>MEAGITGTWY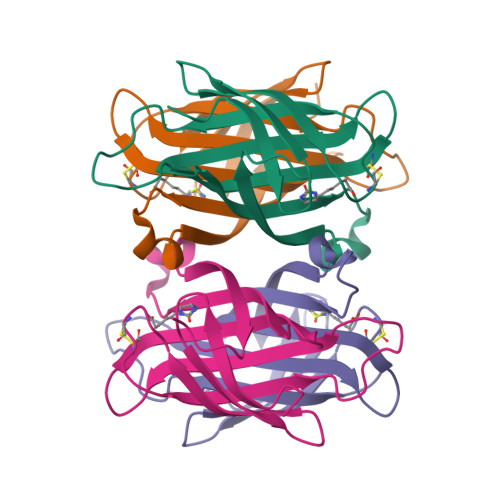NQLGSTFIVTAGADGALTGTYESAVGCAESRYVLTGRYDSAPATDGSGTALGWTVAWKNNYRNCHSATTWSGQYVGGAEARINTQWLLTSGTTEANAWKSTLVGHDTFTKVKPS[12x]First structural insight into lipid scrambling was provided from the X-ray structure of the fungal protein from Nectria haematococca, termed nhTMEM16. This protein is part of the TMEM16 family, which encompasses calcium-activated ion channels and lipid scramblases with a conserved molecular architecture. As common for the family, nhTMEM16 is a homodimer with subunits containing a cytoplasmic domain and a transmembrane unit composed of 10 membrane-spanning segments. The lipid permeation path is defined by a structural entity termed the ‘subunit cavity’, which is located at the periphery of each subunit. The ‘subunit cavity’ is believed to provide a pathway for the polar moieties of lipids across the membrane, whereas the apolar acyl chains remain embedded in the hydrophobic core of the bilayer.

For the structural characterization of nhTMEM16, we have initially studied Ca2+-bound and Ca2+-free samples in detergent by cryo-EM. By this approach, we have obtained two datasets of high quality and of sufficient resolution (i.e. 3.6 Å for Ca2+-bound and 3.7 Å for Ca2+-free conditions) for a detailed interpretation by an atomic model (Figure 1—figure supplements 2–4). In the structure determined in the presence of Ca2+, we find a conformation of the protein, which closely resembles the X-ray structure with a root mean square deviation (RMSD) of Cα atoms of 0.66 Å between the two structures. The high similarity prevails irrespective of the absence of crystal packing interactions and despite of the fact that the sample used for cryo-EM was only briefly exposed to Ca2+ at a comparably low (i.e. 300 µM) concentration, whereas for the X-ray structure, the protein was exposed to Ca2+ during purification and crystallization at a 10-fold higher concentration. Cryo-EM density at the conserved Ca2+-binding site, contained within each subunit of the homodimer, clearly indicates the presence of two bound Ca2+ ions located at the position originally identified in the X-ray structure. Instead, it is likely a consequence of experimental conditions, which stabilize the observed conformation of the protein. This is in accordance with residual density from the headgroup of a bound detergent molecule at the upper part of the lipid translocation path found in both datasets, which might prevent subunit cavity closure. The Ca2+-bound conformation in detergent and the ‘open’ class observed in the data of Ca2+-bound protein in nanodiscs both show the widest opening of the subunit cavity and thus likely depict a scrambling-competent state of the protein. In this open state, α-helices 4 and 6 are separated from each other on their entire length framing the two opposite edges of a semicircular polar furrow that is exposed to the lipid bilayer. On the opposite border of the subunit cavity, α6 is immobilized in its position by the bound Ca2+ ions, which results in a tight interaction with α7 and α8.

>MSNLKDFSQPGSGQESNFGVDFVIHYKVPAAERDEAEAGFVQLIRALTTVGLATEVRHGENESLLVFVKVASPDLFAKQVYRARLGDWLHGVRVSAPHNDIAQALQDEPVVEAERLRLIYLMITKPHNEGGAGVTPTNAKWKHVESIFPLHSHSFNKEWIKKWSSKYTLEQTDIDNIRDKFGESVAFYFAFLRSYFRFLVIPSAFGFGAWLLLGQFSYLYALLCGLWSVVFFEYWKKQEVDLAVQWGVRGVSSIQQSRPEFEWEHEAEDPITGEPVKVYPPMKRVKTQLLQIPFALACVVALGALIVTCNSLEVFINEVYSGPGKQYLGFLPTIFLVIGTPTISGVLMGAAEKLNAMENYATVDAHDAALIQKQFVLNFMTSYMALFFTAFVYIPFGHILHPFLNFWRATAQTLTFSEKELPTREFQINPARISNQMFYFTVTAQIVNFATEVVVPYIKQQAFQKAKQLKSGSKVQEDHEEEAEFLQRVREECTLEEYDVSGDYREMVMQFGYVAMFSVAWPLAACCFLVNNWVELRSDALKIAISSRRPIPWRTDSIGPWLTALSFLSWLGSITSSAIVYLCSNSKNGTQGEASPLKAWGLLLSILFAEHFYLVVQLAVRFVLSKLDSPGLQKERKERFQTKKRLLQENLGQDAAEEAAAPGIEHSEKITREALEEEARQASIRGHGTPEEMFWQRQRGMQETIEIGRRMIEQQLAAGKNGKKSAPAVPSEKAS[2x]The patellamides are eight-residue cyclic peptides containing oxazolines, thiazoles and d-amino acids and are derived from a ribosomally produced precursor peptide. The patellamide gene cluster has been identified (seven genes; patA–patG) and the majority of the proteins or their contributing domains have been assigned specific functions. PatF has been shown to be essential for patellamide production in vivo; however, to date its function has not been confirmed. Cyanobactin family members related to PatF have been shown to possess prenyltransferase activity.

Here, we report the crystal structure of PatF, the first from this cyanobactin enzyme family, to a resolution of 2.1 Å and provide evidence to suggest that it is likely to be an inactive prenyltransferase. The crystal structure of PatF has been solved and comprises a β-­barrel core surrounded by α-helices, which is a known motif for prenyltransferases. PatF is a globular protein with approximate dimensions of 45 × 43 × 53 Å. There is a single disulfide bridge at the C-­terminus linking Cys276 and Cys307. The final refined model contains residues 3–196 and 205–307 of chain A and residues 2–196 and 205–307 of chain B. The missing residues are found on the connecting loop between β8 and α8 and also at the N- and C-termini, all of which are presumed to be disordered. Electrostatic surface-potential representations of PatF highlight a highly electronegative central pore that could disfavour binding of the electronegative DMAPP. Two key interactions of DMATS were identified to involve Lys187 and Asp178, which both play a role in binding DMAPP. In PatF, the structurally equivalent residues to Lys187 and Asp178 are Met136 and His125, respectively. These significant changes mean that Met136 would not form the same salt-bridge interaction as the lysine in DMATS, while His125 would have a repulsive effect on Arg66 (the equivalent of Arg100 in DMATS) rather than a stabilizing interaction. Our data, together with the lack of prenylation of any natural patellamide, indicate that PatF is an inactive prenyltransferase.

>DLIDRLQNNQRKDRRLQFVRTHQEAFDVKPTFPLPLFEEAILEIEGSCSVESSCQVEGDRLQGGRYEVCNNQGTTWPESLTHAFKLLDKIDSQLGVRINRDSFDRFAAAHVNSRKIINNTIGVHLGSKLEDSSVMLYIHIKPEEDTEELARTALVLDGGRYSDELTRVLLRDTMVIGFELFFDGRSRVDLGPCAPGKSGTLKMKGKHLEQYTQKNLSRKVNSIFREGYLFGAFFSKTRVEPILFFYHSIIKDLPKYFTFNSLGDKIYNFCQSQGCITDVAIAVTETELEKSRLENFCFYYDQWDECKPSSDYDTERHLHRS[2x]>[2x]MIFVNDVYKNFGSLEVLKGVTLKVNKGEVVVIIGPSGSGKSTLLRCINLLEEPTKGEVFIDGVKINNGKVNINKVRQKVGMVFQHFNLFPHLTAIENITLAPVKVKKMNKKEAEELAVDLLAKVGLLDKKDQYPIKLSGGQKQRLAIARALAMQPEVMLFD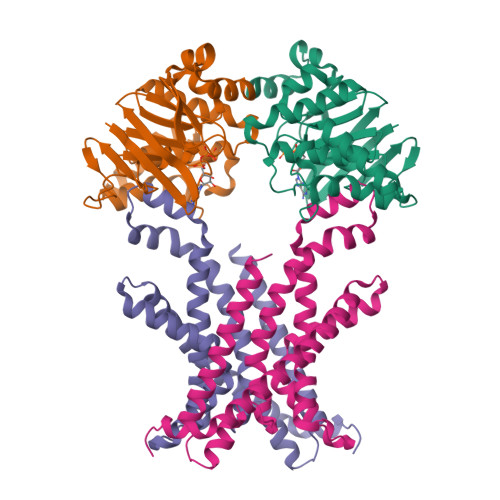EPTSALDPEMVKEVLNVMKQLANEGMTMVVVTHEMGFAREVGDRVIFMDDGVIVEEGTPEEIFYRAKNERTREFLSKIL;>[2x]MTVDFLSMVKYTPLFISGLIMTLKLTFLAVTIGVLMGLFIALMKMSSIKPIKLVASSYIEVIRGTPLLVQLLLIYNGLMQFGMNIPAFTAGVSALAINSSAYVAEIIRAGIQAVDPGQNEAARSLGMTHAMAMRYVIIPQAIKNILPALGNEFIVMLKESAIVSVIGFADLTRQADIIQSVTYRYFEPYIIIAAIYFVMTLTFSKLLSLFERRLRAGDIR>HHHHHHMALQLAAHSDARSGPVGSNGGQFWSFRPVRPLNKIVLSFSGSPDQTLNLISITFSSNPTDIITVGGVGPEPLTYTETVNIDGDIIEISGMIANYKGYNVIRSIKFTTNKKEYGPYGANAGTPFNIKIPDGNKIVGFFGNSGW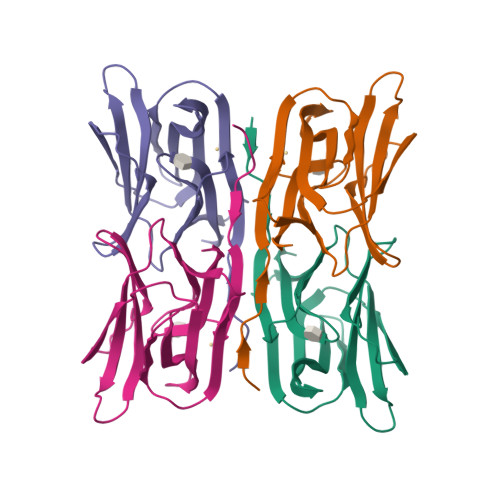YVDAIGAYYTAK[4x]>LNSVGQGEFGGAPFKRFLRGTRIVSGGKLKRMTREKAKQVTVAGVPMPRDAEPRHLLVNGATGTGKSVLLRELAYTGLLRGDRMVIVDPNGDMLSKFGRDKDIILNPYDQRTKGWSFFNEIRNDYDWQRYALSVVPRGKTDEAEEWASYGRLLLRETAKKLALIGTPSMRELFHWTTIATFDDLRGFLEGTLAESLFAGSNEASKALTSARFVLSDKLPEHVTMPDGDFSIRSWLEDPNGGNLFITWREDMGPALRPLISAWVDVVCTSILSLPEEPKRRLWLFIDELASLEKLASLADALTKGRKAGLRVVAGLQSTSQLDDVYGVKEAQTLRASFRSLVVLGGSRTDPKTNEDMSLSLGEHEVERDRYSKNTGKHHSTGRALERVRERVVMPAEIANLPD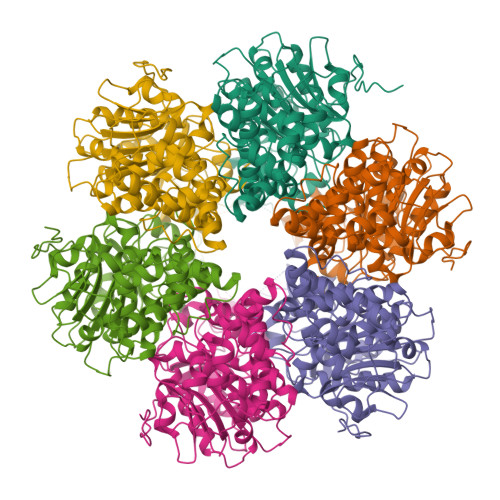LTAYVGFAGNRPIAKVPLEIKQFANRQPAFVEGTI[12x]> AKNLEPVSWSSLNPKFLSGKGLVIYPKIGDKLDIICPRAEAGRPYEYYKLYLVRPEQAAACSTVLDPNVLVTCNKPHQEIRFTIKFQEFSPN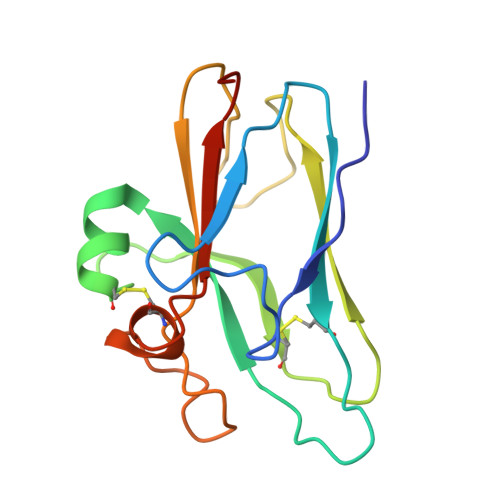YMGLEFKKYHDYYITSTSNGSLEGLENREGGVCRTRTMKIVMKVGQDPNA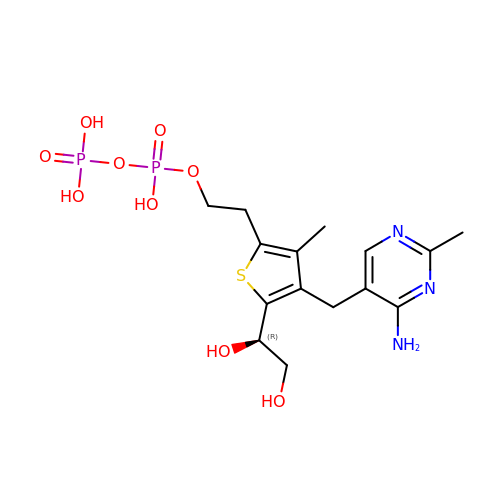2-{4-[(4-amino-2-methylpyrimidin-5-yl)methyl]-5-[(1R)-1,2-dihydroxyethyl]-3-methylthiophen-2-yl}ethyl trihydrogen diphosphate | C15 H23 N3 O9 P2 S | AZNRIYLXMXTRTE-GFCCVEGCSA-N> MQHNAEAAAAAESSTSTVSNLATMATVTASGREVSSGFGPELAADNQDLPDNPTDKSVHNASGASRWSADRGSGPWWLAYEFPGEATISSVNIAWGNTYATNYSIQTSDDGSNWTDVKTGLKATAQAQWVKTTFDTPIKTRHIRMIATTKSQSWSLSVWEMRTMGTISAVATDPLSRLTPRPLYAQSADGEAFELKKNTCVSVSDGSLLPAVDVMRDELGTSYGLKLAEGTNCPITFTLDENLDVTGHVGSAQSITADEAYTIVSDADSVTVKARSATAGIWAAQTLLQLIGPWTNSTVKLADVAFIPAVNIADAPRYQWRGVLVDPARSFYPLDEMKQMIDVMSAYKMNTLHLHLSEDEGFRVEITNDGRADGDTTDYTQLAIKSGAISYQSAWTSNWSPAQDGRTGYWTQSEFIELVAYAADHGIAIVPEIDGPGHSFSLLHGLAELNTGNSNPKPAAGEDTPAFIQSAQGRSSLATDADITYTVLGHIMDQLDGMIDKGIKASTMPASELKRMYFHLGGDELFLSGGAGNKTERLQEYLGRSGALVKERDKTTIVWNDGLDAVDQIPEGSVVQHWTGNAANNASIQKLLNQRNGKIIMSPAGNTYFPQRPGTETTGVTWACGACTTSNFYQWNPTSSAGTTEDKVLGVEDALWSEHLRSLNDAEFLMYTRMMATAEVGWTQQNRKDYDNWNKRVGDIAIDLMNRGANFHKATEVTSWKGSYAAVDAAEQKVTDGKVLVGRYAEPGLTGTDGLSFTATYTAEGGTAVNLPVTPDMKQTYSQQQLKNGRLVVNGAHMNSIVDVYVTLPSDVLAADSE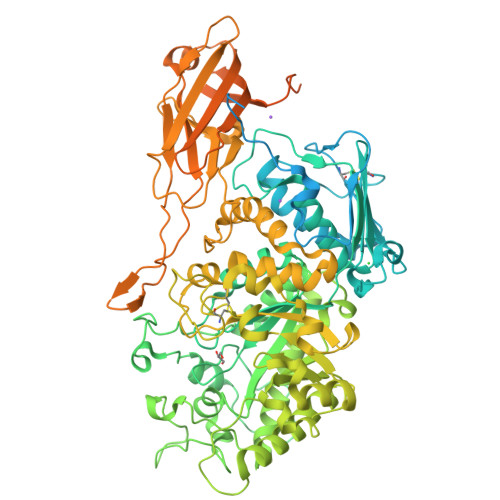AVGRLDVSVSSSTYPIPSDSSMSIAIKDGKVTQTWTGDERPTPDPDPEPEVTVVSIKASTSQSDVKVGDTFDPSKVKVVATKSDKTTAVLAAADYTIAVTDKDGNAIDVTKPFEAAGDLTVTVALKDDGSIKDSFTMTVTDKGAVDPDPDPTPKPNPDPQKPSGDNKPQIKPEGGKPGDVVAETLEHHHHHH The non-structural protein 1 (NS1) is secreted from the infected cell and is thought to be associated with disease severity besides its proven usefulness for differential diagnoses. NS1 can be found intracellularly, where it is essential for virus replication, docked on lipid rafts of the cell surface membrane, and abundantly secreted into the bloodstream of infected individuals during the febrile phase. NS1 is comprised of three distinct domains, an N-terminal hydrophobic β-roll dimerization domain (residues 1–29) formed by the intertwining of two protomers, an α/β-wing domain (residues 38–151) that extends out from the central β-ladder domain (residues 181–352) giving the dimer a distinct crossed shape. Here, we present high-resolution cryoEM structures of ZIKV recombinant secreted NS1 (rsNS1) and its complexes with three human monoclonal antibodies (AA12, EB9, GB5), as well as evidence for ZIKV infection-derived secreted NS1 (isNS1) binding to High Density Lipoprotein (HDL).

Unexpectedly, we observed that ZIKV rsNS1 forms filaments. Subsequent helical reconstruction of ZIKV rsNS1 filaments resulted in a low-resolution map of 8 Å, which could be fitted with ZIKV rsNS1 dimers. These ZIKV rsNS1 filaments are flexible and composed of asymmetric tetramers (dimer pairs) stacked along their exposed wing-ladder domain surfaces which possess complementary electrostatic surfaces. In addition, ZIKV rsNS1 at a lower concentration forms a filamentous chain driven largely by the complementary surface charge interactions of the wing ladder. Here, we provide further evidence that the recombinant, secreted ZIKV NS1 forms tetramers with a distinct ability to oligomerize into filamentous structures. While the potential pathophysiological implications of rsNS1 filaments or microtubules are unclear and could simply be induced by the in vitro environment, such structures, as previously observed by us28 and others, highlight discrepancies regarding the true soluble form of oligomeric NS1.

>[10x]DVGCSVDFSKKETRCGTGVFIYNDVEAWRDRYKYHPDSPRRLAAAVKQAWEEGICGISSVSRMENIMWKSVEGELNAILEENGVQLTVVVGSVKNPMWRGPQRLPVPVNELPHGWKAWGKSYFVRAAKTNNSFVVDGDTLKECPLEHRAWNSFLVEDHGFGVFHTSVWLKVREDYSLECDPAVIGTAVKGREAAHSDLGYWIESEKNDTWRLKRAHLIEMKTCEWPKSHTLWTDGVEESDLIIPKSLAGPLSHHNTREGYRTQVKGPWHSEELEIRFEECPGTKVYVEETCGTRGPSLRSTTASGRVIEEWCCRECTMPPLSFRAKDGCWYGMEIRPRKEPESNLVRSMVTAHHHHHH One such T6SS effector is Tlde1a from Salmonella Typhimurium. Tlde1a functions as an LD-carboxypeptidase to cleave tetrapeptide stems and as an LD-transpeptidase to exchange the terminal D-alanine of a tetrapeptide stem with a noncanonical D-amino acid. Our structural data revealed that Tlde1a possesses a unique LD-transpeptidase fold consisting of a dual pocket active site with a capping subdomain. This includes an exchange pocket to bind a D-amino acid for exchange and a catalytic pocket to position the D-alanine of a tetrapeptide stem for cleavage.

To probe the molecular features of Tlde1a that may contribute to this activity, we soaked Tlde1a crystals with D-Ala and D-Met. We were able to obtain cocrystal structures of Tlde1a in complex with each amino acid. The interaction of both D-amino acids with Tlde1a is facilitated by a salt bridge between the D-amino acid carboxylic acid and the sidechain of R115. Interestingly, the hydrophobic sidechain of D-Met faces toward the solvent and has no significant interaction with the active site of Tlde1a. Although the His-tag is an artifact, binding of the known D-Met substrate to Tlde1a induces a drastic conformational change in the His-tag. Compared to the native and D-Ala–bound structures, the His-tag in the D-Met–bound structure has significantly shifted its position within the Tlde1a active site. This change also includes the ability to model five His-tag residues instead of four and the loss of two ordered sulfates. Additionally, the binding of D-Met and the reordering of the His-tag induces a conformational change in the Tlde1a capping subdomain relative to both the sulfate and D-Ala–bound structures. Given the observed His-tag peptide bound in the active site of Tlde1a and that both the artifact and the capping subdomain change conformation upon binding of D-Met, we hypothesize that like YcbB the capping subdomain of Tlde1a stabilizes a peptide stem for transpeptidase exchange activity and potentially for crosslinking.

> MAVRLTFDGQKLTWPGIGIFKATTGLPDLQWPDKQCVPDAAIPEGNYKLFIQFQGEAPIRNAADCDLGPSWGWSTIPRGQAAGTCEIYWANWGYNRIRLESADEKTRKACGGKRGGFYIHDSTKGYSHGCIEVEPVFFRILKQETEKENGEKTFTVNVKYVSGQQTNGGTKQGE;> HHHHHH>AAHHSSGHMEATLGSGNLRQAVMLPEGEDLNEWIAVNTVDFFNQINMLYGTITEFCTEASCPV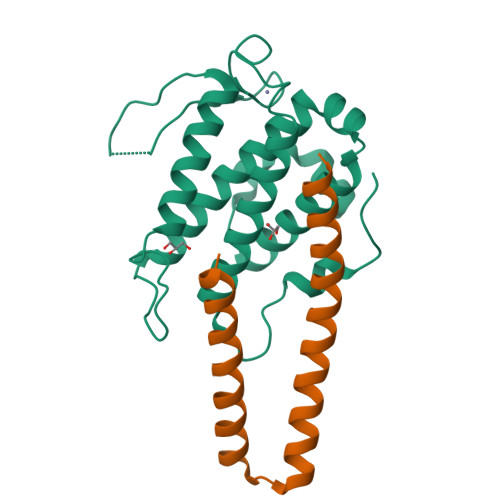MSAGPRYEYHWADGTNIKKPIKCSAPKYIDYLMTWVQDQLDDETLFPSKIGVPFPKNFMSVAKTILKRLFRVYAHIYHQHFDSVMQLQEEAHLNTSFKHFIFFVQEFNLIDRRELAPLQELIEKLGSKDR[2x];>[2x]SSGHMKLTLENFYSNLILQHEERETRQKKLEVAMEEEGLADEEKKLRRSQHARKETEFLRLKRTRLGL> SERDKKELVNAIEDRAACFLTKQWSLSPIGSAVPGTRTVAILCCQETADLAAEVSSYFPNHLLIDVSRIENDQSDIDWKEFDGLVDVIGCGWDDEGRLDWIEWVQRLVEFGHKEGLRLLCVTKGLESFQNTSVRMAGASRAGLYRMLQCEYSHLISRHMDAEEVTDHRRLAKLIADEFYSDSYDAEVCYRDGLRYQAFLKAHPETGKATEQSAVFPKDHVLLITGGTRGIGLLCARHFAECYGVKKLVLTGREQLPPREEWARFKTSNTSLAEKIQAVRELEAKGVQVEMLSLTLSDDAQVEQTLQHIKRTLGPIGGVIHCAGLTDMDTLAFIRKTSDDIQRVLEPKVSGLTTLYRHVCNEPLQFFVLFSSVSA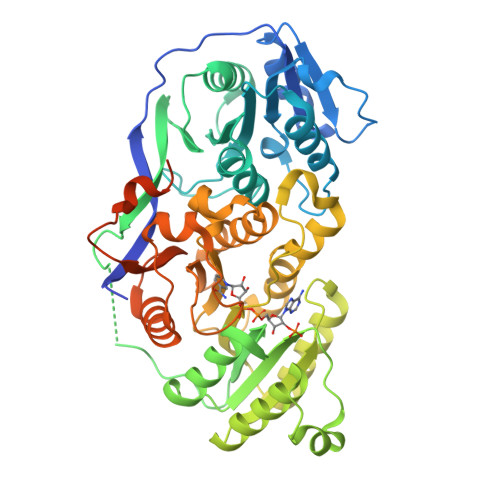IIPELSAGQADYAMANSYMDYFAEAHQKHAPIISVQWPNWKETGMGEVTNQAYRDSGLLSITNSEGLRFLDQIVSKKFGPVVLPAMANQTNWEPELLMKRRKPHEGGLQEAALQSPPARDIEEADEVSKCDGLLSETQSWLIDLF Here, we report evidence that MBLAC1 is a nuclease specific for cleavage of RD histone pre-mRNA. Crystallographic and biochemical studies show that MBLAC1 has an overall MBL fold and di-zinc ion containing active site related to that of CPSF73, but which has distinctive structural features involving active site flanking loops and the absence of the β-CASP domain, which is only present in CPSF73. The combined biochemical, cellular, and genetic analyses presented here provide clear evidence that MBLAC1 is an endoribonuclease selective for 3' end processing of RD histone pre-mRNA during S-phase of the cell cycle. Studies with recombinant MBLAC1 purified from human or E. coli cells, define MBLAC1 as an endoribonuclease, with selectivity for cleavage at the biologically authentic CA dinucleotides (positions 27 and 29 using our nomenclature).

To investigate its function, we solved a crystal structure of MBLAC1 (1.8 Å resolution, space group P1). The structure reveals a stereotypical αββα MBL- fold with two central mixed β-sheets (I and II), comprised of 8 and 5 strands respectively, surrounded by helices. MBLAC1 has four of the five characteristic MBL-metal-binding motifs, His116, His118 Asp120 and His121 (motif II), His196 (motif III), Asp221 (motif IV) and His263 (motif V) (using BBL numbering) with two waters completing metal coordination. In the structure of recombinant MBLAC1 produced in E. coli, the active site was refined with two iron ions present. However, MBLAC1 produced in HEK293 cells preferentially binds zinc ions. Four MBLAC1 molecules (chains A-D) are present in the crystallographic asymmetric unit; analysis of interactions at the crystallographically observed monomer interfaces identified interactions between chains A-B and C-D possibly reflecting dimeric MBLAC1 in solution. The metal containing active site is adjacent to the dimer interface, rationalizing reduced dimerization as manifested by metal ligand substitution or metal removal. However, although there is low overall sequence similarity (27%), the overall MBLAC1 fold is structurally similar to the human endoribonuclease β-lactamase-like-protein 2 (LACTB2), RMSD 2.23 Å over 153 Cα atoms, an endoribonuclease responsible for mitochondrial mRNA maturation. Comparison of the MBLAC1 and LACTB2 active sites reveals very similar di-metal ion binding modes and proximate active site residues. Two other regions in the MBLAC1 structure (aa 51–66 and the C-terminal region, aa 239–266) are disordered, implying flexibility and possible involvement in substrate recognition.

>MRTEPLCGASPLLVPGDPYSVVVLLQGYAEPEGVGDAVRADGSVTLVLPQTRGPASSHRESPRGSGGAEAALEEAARGPILVDTGGPWAREALLGALAGQGVAPGDVTLVVGTHGHSDHIGNLGLFPGAALLVSHDFCLPGGRYLPHGLGEGQPLRLGPGLEVWATPGHGGQRDVSVVVAGTALGTVVVAGDVFERDGDEDSWQALSEDPAAQERSRKRVLVVADVVVPGHGPPFRVLREASQPETEGGGNSQQEPVVGDEEPALH[4x]> GHMSNTSWRKSEVLAVPLQPTLQQEVILARMEQILASRALTDDERAQLLYERGVLYDSLGLRALARNDFSQALAIRPDMPEVFNYLGIYLTQAGNFDAAYEAFDSVLELDPTYNYAHLNRGIALYYGGRDKLAQDDLLAFYQDDPNDPFRSLWLYLAEQKLDEKQAKEVLKQHFEKSDKEQWGWNIVEFYLGNISEQTLMERLKADATDNTSLAEHLSETNFYLGKYYLSLGDLDSATALFKLAVANN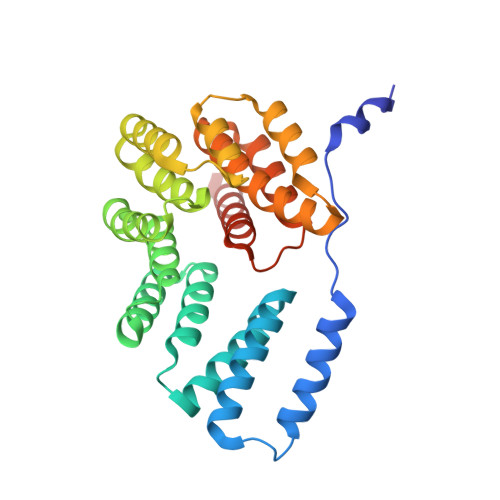VHNFVEHRYALLELSLLGQDQDDLAESDQQ> MPK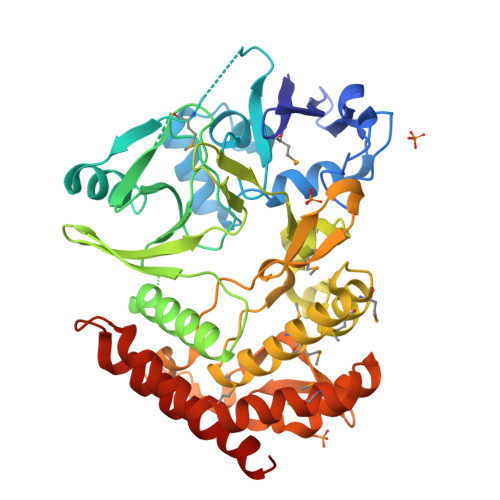LVTWMNNQRVGELTKLANGAHTFKYAPEWLASRYARPLSLSLPLQRGNITSDAVFNFFDNLLPDSPIVRDRIVKRYHAKSRQPFDLLSEIGRDSVGAVTLIPEDETVTHPIMAWEKLTEARLEEVLTAYKADIPLGMIREENDFRISVAGAQEKTALLRIGNDWCIPKGITPTTHIIKLPIGEIRQPNATLDLSQSVDNEYYCLLLAKELGLNVPDAEIIKAGNVRALAVERFDRRWNAERTVLLRLPQEDMCQTFGLPSSVKYESDGGPGIARIMAFLMGSSEALKDRYDFMKFQVFQWLIGATQGHAKNFSVFIQAGGSYRLTPFYDIISAFPVLGGTGIHISDLKLAMGLNASKGKKTAIDKIYPRHFLATAKVLRFPEVQMHEILSDFARMIPAALDNVKTSLPTDFPENVVTAVESNVLRLHGRLSREYGSK The Vtc4p β-tunnel domain is not unique to eukaryotic polyP polymerases but is a structural hallmark of triphosphate tunnel metalloenzymes (TTMs), whose characteristic features are the presence of a topologically closed hydrophilic β-barrel, the preference for triphosphate-containing substrates, and for a divalent metal co-factor (PFAM families CYTH and VTC). Members of the ancient triphosphate tunnel metalloenzyme family can be found in all kingdoms of life. Our comparative analysis defines that most of these enzymes share a common catalytic mechanism in their tunnel centers, yet they have evolved different substrate recognition modes on their tunnel entries. The observed substrate plasticity apparently allows TTM proteins to act on a wide array of enzyme substrates and to perform very different reactions, many of which likely remain to be discovered.

Instead, AtTTM3 has specific, Mg2+ ion-dependent, short-chain polyphosphatase activity as previously reported. As AtTTM3 efficiently hydrolyzes PPPi in the presence of Mg2+ ions only at neutral or basic pH, we used two crystal forms grown at pH 5.0 (form A) and pH 7.5 (form B) to crystallize substrate-metal complexes under non-hydrolyzable and hydrolyzable conditions, respectively. In both crystal forms, we determined structures of AtTTM3 in the presence of PPPi and either MgCl2 or MnCl2. At pH 5.0 (form A) we find a triphosphate moiety bound in the AtTTM3 active site. Here, PPPi coordinates a Mg2+/Mn2+ ion that acts as a bridge between the substrate and the invariant Glu-169AtTTM3. The same metal co-factor coordination has been previously found in a Vtc4p AppNHp-Mn2+ complex. Here, the octahedral coordination of the Mg2+/Mn2+ ion is completed by an glutamate residue (Glu-169AtTTM3, Glu-160ygiF), which is invariant in all TTM proteins characterized thus far.

>GAMEVEVKLRLLTAAAHLRLTTLLTPYHLKTLHQRNTFFDTPKNDLSLRRAVLRLRFLQNAAVSAASPSPPRCIVSLKAKPTLANGISRVEEDEEEIEYWIGKECVESPAKLSDIGSRVLKRVKEEYGFNDFLGFVCLGGFENVRNVYEWRGVKLEVDETKYDFGNCYEIECETEEPERVKTMIEEFLTEEKIEFSNSDMTKFAVFRSGKLP[2x]>MSDKDSKNTPQVPEKLGLSRRGFLGASAVTGAAVAATALGGAVMTRESWAQAVKESKQKIHVGPGELDDYYGFWSGGHQGEVRVLGVPSMRELMRIPVFNVDSATGWGLTNESRHIMGDSAKFLNGDCAHPHISMTDGKYDGKYLFINDKANSRVARIRLDIMKCDKMITVPNVQAIHGLRLQKVPHTKYVFANAEFIIPHPNDGKVFDLQDENSYTMYNAIDAETMEMAFQVIVDGNLDNTDADYTGRFAAATCYNSEKAFDLGGMMRNERDWVVVFDIHAVEAAVKAGDFITLGDSKTPVLDGRKKDGKDSKFTRYVPVPKNPHGCNTSSDGKYFIAAGKLSPTCSMIAIDKLPDLFAGKLADPRDVIVGEPELGLGPLHTTFDGRGNAYTTLFIDSQVVKWNMEEAVRAYKGEKVNYIKQKLDVHYQ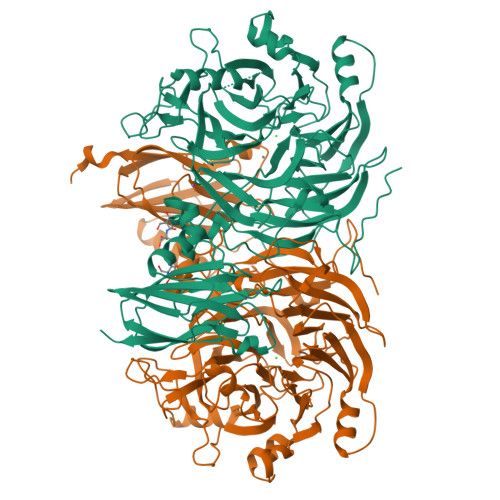PGHLHASLCETNEADGKWLVALSKFSKDRFLPVGPLHPENDQLIDISGDEMKLVHDGPTFAEPHDCIMARRDQIKTKKIWDRNDPFFAPTVEMAKKDGINLDTDNKVIRDGNKVRVYMTSMAPAFGVQEFTVKQGDEVTVTITNIDQIEDVSHGFVVVNHGVSMEISPQQTSSITFVADKPGLHWYYCSWFCHALHMEMVGRMMVEPAWSHPQFEK[2x]S-1,2-PROPANEDIOL | C3 H8 O2 | 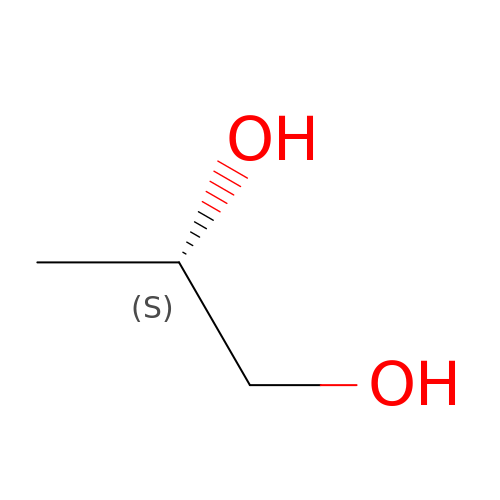DNIAPMSPPWPWGF-VKHMYHEASA-N>[2x]GSMTVLQEPVQAAIWQALNHYAYRDAVFLAERLYAEVHSEEALFLLATCYYRSGKAYKA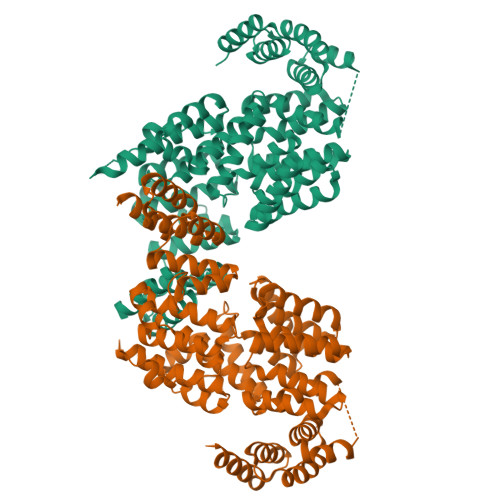YRLLKGHSCTTPQCKYLLAKCCVDLSKLAEGEQILSGGVFNKQKSHDDIVTEFGDSACFTLSLLGHVYCKTDRLAKGSECYQKSLSLNPFLWSPFESLCEIGEKPDPDQTFKFTSLQNFSNCLPQIQAFNLQKAAAEGLMSLLREMGKGYLALCSYNCKEAINILSHLPSHHYNTGWVLCQIGRAYFELSEYMQAERIFSEVRRIENYRVEGMEIYSTTLWHLQKDVALSVLSKDLTDMDKNSPEAWCAAGNCFSLQREHDIAIKFFQRAIQVDPNYAYAYTLLGHEFVLTEELDKALACFRNAIRVNPRHYNAWYGLGMIYYKQEKFSLAEMHFQKALDINPQSSVLLCHIGVVQHALKKSEKALDTLNKAIVIDPKNPLCKFHRASVLFANEKYKSALQELEELKQIVPKESLVYFLIGKVYKKLGQTHLALMNFSWAMDLDPKGANNQIKEAIDKRYLPDDEEPITQEEQIMGTDESQESSMTDADDTQLHAAESDEF>[3x]HHHHHQSEFIKDSKASIELRNFYFNRDFRQEGASQSKAEEWAQGFLLRYESGYTEGTIGFGVDAIGLLGVKLDSSPDRSGTGLLKRDRETGRAQDDYGEAGITAKLRASKSTLKIGTLTPKLPVIMPNDSRLLPQTFQGGALNSMEIDGLTLDAGRLKKVNQRDSSDNEDMTITGGGKRQIVVRSGLTSDKFDFAGGSYKWTDNLSTSYHYGKLDNFY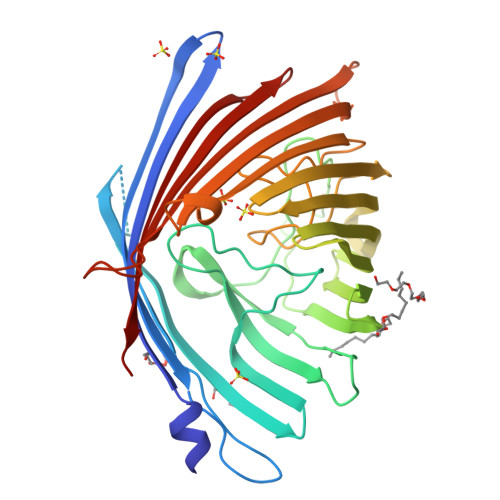KQHYLGLVHTLPIADKQSLKSDIRWARSTDDGSSNVDNKALNAMFTYSLGYHAFGVGYQKMSGDTGFAYINGADPYLVNFIQIGDFANKDEKSWQARYDYNFAGVGIPGLTFMTRYVKGDNIDLLTTSGEGKEWERDMDIAYVFQSGPLKNLGVKWRNATMRTNYTNDYDENRLIVSYTLPLW> GGGDRRKEMDKVYRTAFKRITSTPDKEKRKEVVKEATEQLRRIAKDEEEKKKAA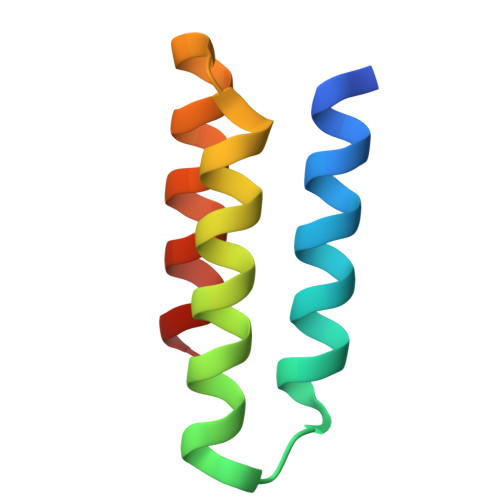YMILFLKTLG Utilizing the published genome sequence of the organism, we hypothesized that the genes 0612, 0638, and 0637 encode for a 4,6-dehydratase, an aminotransferase, and an N-acetyltransferase, respectively, which would be required for the biosynthesis of one of the diacetamido-sugars, 2,4-diacetamido-2,4,6-trideoxy-d-glucose, starting from UDP-N-acetylglucosamine. In this report we present functional and structural data that demonstrate the proteins encoded by the 0638 and 0637 genes do indeed correspond to an aminotransferase (hereafter referred to as Pcryo_0638) and an N-acetyltransferase (Pcryo_0637). In summary, we have demonstrated that the genes in P. cryohalolentis, namely 0638 and 0637, encode for a PLP-dependent aminotransferase and an N-acetyltransferase, respectively. The data presented herein confirm the hypothesized functions of these enzymes and provide new insight into an unusual sugar biosynthetic pathway in Gram-negative bacteria.

An X-ray crystallographic structure of 0638, determined in its external aldimine form to 1.3 Å resolution, demonstrated the manner in which the UDP ligand is positioned into the active site. Crystals of Pcryo_0638 were grown in the presence of PLP and UDP-2-acetamido-4-amino-2,4,6-trideoxy-d-glucose (the product). They belonged to the triclinic space group P1 with a complete dimer in the asymmetric unit. Given that the crystals were grown in the presence of PLP and the product, initial inspection of the map suggested that the external aldimine was bound. Even after modeling the ligand into the map, however, there was residual electron density calculated with (Fo–Fc) coefficients. To account for this observation, a mixture of the external aldimine and PMP was subsequently built into the electron density with each given half-occupancy. The uracil ring, however, is sandwiched between the side chains of Phe 335 and Tyr 229, which is contributed by subunit B. There are two additional interactions between it and the backbone amide of Gly 337 and an ordered water molecule. The side chains of Tyr 229 and Lys 215, both contributed by subunit B, lie within 3.2 Å of an α- and a β-phosphoryl oxygen, respectively. The C-2' acetamido group is anchored into the active site by the side chain of Gln 183 and a water molecule, whereas the pyranosyl ring oxygen lies at 3.0 Å from a water molecule. Whereas both enzymes function on the same substrate, the manner in which the ligands are accommodated in the active sites is remarkably different.

>GGGHMLNTPFSPWPSFTQIEADAVSRVLLSNQVNYWTGQECRQFETEFAEWADSKYAIAMGNGTLALDVALQALDIGAGDEVIVTPRTFIASISSVVNIGATPVFSDVDEATGNITPESIAAVLTDKTKGIVCVHLAGWPCDMDGIMALADKHNLYVIEDCAQAHGATYKGRSVGSIGHIGAWSFCQDKIMTTGGEGGMVTTNDEQLWRKMWAYKDHGKSYAAVYETDHAPGYRWLHESFGTNWRMTEMQAVLGRIQLKRMPDWTAKRTANAQTILDACAKWEAKGYLSVPRLEESVQFADSTHAYYKLYVYVQSDNLPKEWSRDRIIREINDLGVPCFSGSASEVYLEKAFDNTGLRPENRLPVAKQLGETSLMFLVHPTLTEDEIKQTVQAIDGVFANIHNQ[2x]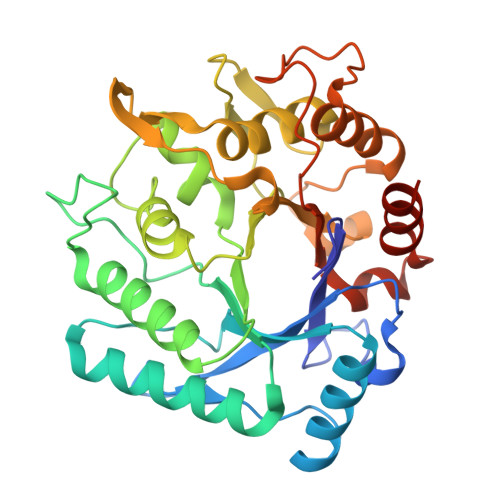> ANNLGSKLLVGYWHNFDNGTGIIKLKDVSPKWDVINVSFGETGGDRSTVEFSPVYGTDADFKSDISYLKSKGKKVVLSIGGQNGVVLLPDNAAKDRFINSIQSLIDKYGFDGIDIDLESGIYLNGNDTNFKNPTTPQIVNLISAIRTISDHYGPDFLLSMAPETAYVQGGYSAYGSIWGAYLPIIYGVKDKLTYIHVQHYNAGSGIGMDGNNYNQGTADYEVAMADMLLHGFPVGGNANNIFPALRSDQVMIGLPAAPAAAPSGGYISPTEMKKALNYIIKGVPFGGKYKLSNQSGYPAFRGLMSWSINWDAKNNFEFSNNYRTYFDGLSLQK> MEHVAFGSEDIENTLAKMDDGQLDGLAFGAIQLDGDGNILQYNAAEGDITGRDPKQVIGKNFFKDVAPXTD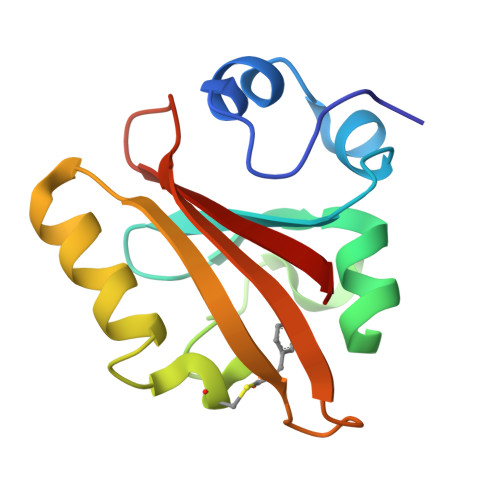SPEFYGKFKEGVASGNLNTMFEYTFDYQMTPTKVKVHMKKALSGDSYWVFVKRV>[2x]MQKPVCLVVAMTPKRGIGINNGLPWPHLTTDFKHFSRVTKTTPEEASRLNGWLPRKFAKTGDSGLPSPS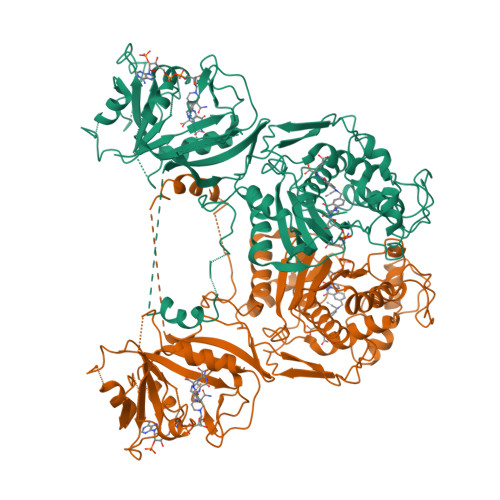VGKRFNAVVMGRKTWESMPRKFRPLVDRLNIVVSSSLKEEDIAAEKPQAEGQQRVRVCASLPAALSLLEEEYKDSVDQIFVVGGAGLYEAALSLGVASHLYITRVAREFPCDVFFPAFPGDDILSNKSTAAQAAAPAESVFVPFCPELGREKDNEATYRPIFISKTFSDNGVPYDFVVLEKRRKTDDAATAEPSNAMSSLTSTRETTPVHGLQAPSSAAAIAPVLAWMDEEDRKKREQKELIRAVPHVHFRGHEEFQYLDLIADIINNGRTMDDRTGVGVISKFGCTMRYSLDQAFPLLTTKRVFWKGVLEELLWFIRGDTNANHLSEKGVKIWDKNVTREFLDSRNLPHREVGDIGPGYGFQWRHFGAAYKDMHTDYTGQGVDQLKNVIQMLRTNPTDRRMLMTAWNPAALDEMALPPCHLLCQFYVNDQKELSCIMYQRSCDVGLGVPFNIASYSLLTLMVAHVCNLKPKEFIHFMGNTHVYTNHVEALKEQLRREPRPFPIVNILNKERIKEIDDFTAEDFEVVGYVPHGRIQMEMAV Here, we report the crystal structures of PstA from L. monocytogenes (LmPstA) bound to c-di-AMP and in the apo form. On the basis of these observations, we conclude that PstA is related to the larger PII protein superfamily, but has diverged through evolution to specifically recognize the bacterial second messenger c-di-AMP and thus is structurally and functionally distinct from the canonical PII proteins. The structure of each LmPstA monomer is composed of a four-stranded antiparallel β-sheet packed against two α-helices on one face. In the LmPstA trimer, the β-sheet of the three monomers form the core, and the α-helices are on the periphery.

We also determined the apo structure of LmPstA at 2.9 Å resolution. There is a trimer of LmPstA in the asymmetric unit for both crystals, and LmPstA migrated as a trimer on a gel filtration column. In the apo LmPstA structure, all of the T-loops and B-loops have disordered regions. The overall structure of the c-di-AMP-bound form of the LmPstA trimer is almost identical to the apo structure with an r.m.s. distance of 0.6 Å for their Cα atoms when they are overlaid. However, there are significant differences in the conformations of the T-loop and B-loop between the apo and c-di-AMP-bound structures. In the apo LmPstA structure, the T-loop from residues 33–39 are largely disordered, indicating that this loop is flexible in the absence of c-di-AMP binding. The C-terminal His-tag of the apo LmPstA structure forms β-sheet interactions with the B-loop, possibly affecting its conformation.

>MKLIFAIVQDQDSNRLSDALTKGNFGATKLATTGGFLKAGNTTFIIGTEDERVEDALAIIKENCKAREQMMTPSASLGVTVDTYVPYPIEVQVGGATVFVMPVESFHHFLEHHH[3x]> MKVYITYGTADFLKT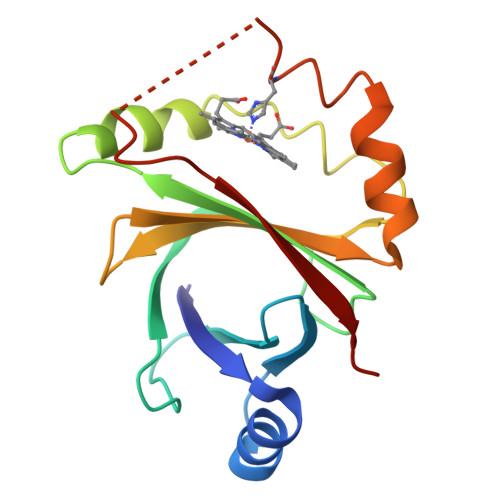IVKKHPSENILLMQGQENAILIHETSGDTVFQAPHAYEVIDQVGEIKHPGFAVLNNIAVTQEGRPLFENKFKNRAGKVENEPGFEAIRVLRPLDSDTYVILTLWETERAFQDWQQSDSYKEAHKKIFSRPSYVTTYFAVE>MVPISPIETVPVKLKPGMDGPKVKQWPLTEEKIKALVEICTEMEKEGKISKIGPENPYNTPVFAIKKKDSTKWRKLVDFRELNKRTQDFWEVQLGIPHPAGLKKKKSVTVLDVGDAYFSVPLDEDFRKYTAFTIPSINNETPGIRYQYNVLPQGWKGSPAIFQSSMTKILEPFKKQNPDIVIYQYMDDLYVGSDLEIGQHRTKIEELRQHLLRWGLTTPDKKHQKEPPFLWMGYELHPDKWTVQPIVLPEKDSWTVNDIQKLVGKLNWASQIYPGIKVRQLSKLLRGTKALTEVIPLTEEAELELAENREILKEPVHGVYYDPSKDLIAEIQKQGQGQWTYQIYQEPFKNLKTGKYARMRGAHTNDVKQLTEAVQKITTESIVIWGKTPKFKLPIQKETWETWWTEYWQATWIPEWEFVNTPPLVKLWYQLEKEPIVGAETFYVDGAANRETKLGKAGYVTNKGRQKVVPLTNTTNQKTELQAIYLALQDSGLEVNIVTDSQYALGIIQAQPDKSESELVNQIIEQLIKKEKVYLAWVPAHKGIGGNEQVDKLVSAG[2x];>GPISPIETVPVKLKPGMDGPKVKQWPLTEEKIKALVEICTEMEKEGKISKIGPENPYNTPVFAIKKKDSTKWRKLVDFRELNKRTQDFWEVQLGIPHPAGLKKKKSVTVLDVGDAYFSVPLDEDFRKYTAFTIPSINNETPGIRYQYNVLPQGWKGSPAIFQSSMTKILEPFKKQNPDIVIYQYMDDLYVGSDLEIGQHRTKIEELRQHLLRWGLTTPDKKHQKEPPFLWMGYELHPDKWTVQPIVLPEKDSWTVNDIQKLVGKLNWASQIYPGIKVRQLSKLLRGTKALTEVIPLTEE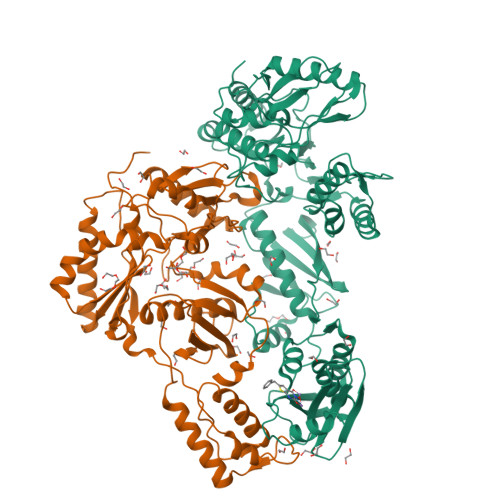AELELAENREILKEPVHGVYYDPSKDLIAEIQKQGQGQWTYQIYQEPFKNLKTGKYARMRGAHTNDVKQLTEAVQKITTESIVIWGKTPKFKLPIQKETWETWWTEYWQATWIPEWEFVNTPPLVKLWYQ[2x]>[30x]MGSSHHHHHHSSGENLYFQGSHMGGIEVLDVKTGPDSTTTIEAYLNPRVGQNWGFSTEITVASNGYNDAPHLTEIPCYSSARISLPLLNEDITSPTLLMWEAVSVKTEVVGISSMLNMHSYGLRAFGGYGGGYTIEGSHIHFFSVGGEPLDLQGLMQNHSTQ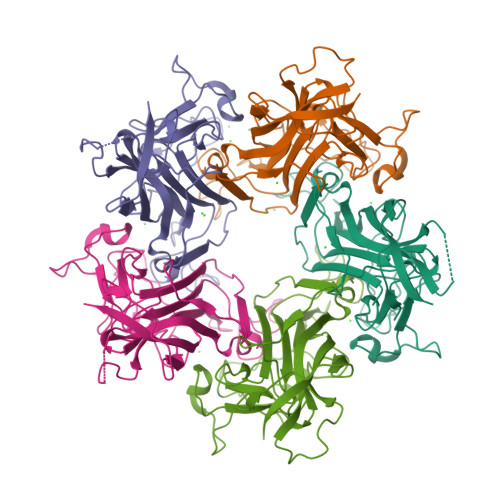YPSPLVGPKKPDGTTDDSAQVLNPIYKAKLDKDATYPIECWCPDPSRNENSRYFGSYTGGVETPPVLSFTNTSTTILLDENGVGPLCKGDGLYLSSADVAGTFVQQTSQKQYWRGLPRYFNITLRKRAVKN> GPGLKQKIVIKVAMEGNNCR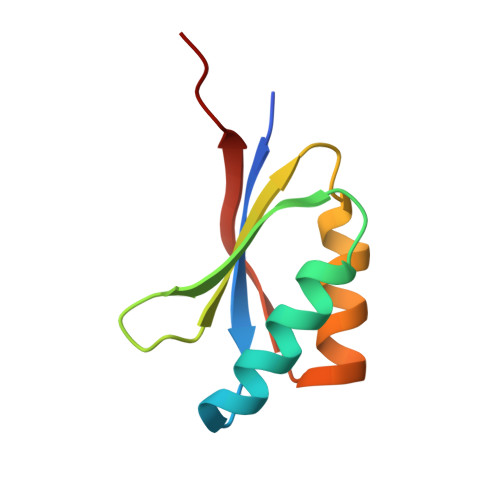SKAMALVASTGGVDSVALVGDLRDKIEVVGYGIDPIKLISALRKKVGDAELLQVSQAKED>AGGKVTSSTGIAPKRYVYYPGSEELGPDEIRVIACGTGMPTARRAQAAAAWVVELGNGDKFIVDIGSGSMANIQSLMIPANYLTKIFLTHLHTDHWGDLVSMWAGGWTAGRTDPLEVWGPSGSREDMGTKYAVEHMLKAYNWDYMTRAVTINPRPGDINVHEFDYRALNEVVYQENGVTFRSWPCIHAGDGPVSFALEWNGYKVVFGGDTAPNIWYPEYAKGADLAIHECWMTSDQMMTKYNQPAQLALRINLDFHTSAQSFGQIMNMVQPRHAVAYHFFNDDDTRYDIYTGVRENYAGPLSMATDMMVWNITRDAVTERMAVSPDHAWDVAGPSEDLAPDRNRASEYT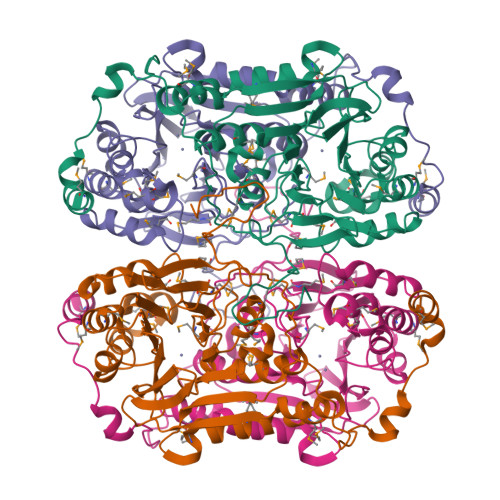QYILDGRLNVDEANAHWKQEFMG[8x]> GAMIRSRQPLLDALGVDLPDELLSLALTHRSYAYENGGLPTNERLEFLGDAVLGLTITDALFHRHPDRSEGDLAKLRASVVNTQALADVARRLCAEGLGVHVLLGRGEANTGGADKSSILADGMESLLGAIYLQHGMEKAREVILRLF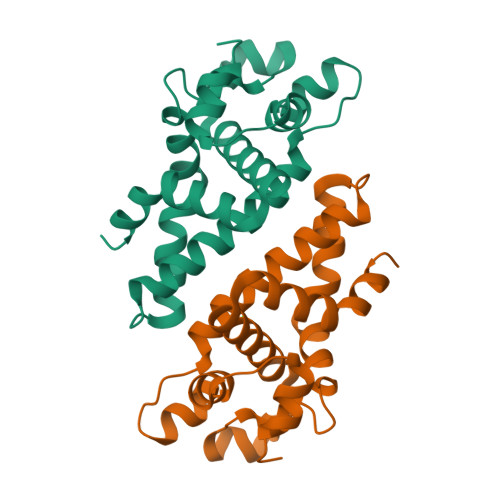GPLLDAAPTLGAGLDWKTSLQELTAARGLGAPSYLVTSTGPDHDKEFTAVVVVMDSEYGSGVGRSKKEAEQKAAAAAWKALEVLDNAMPGKTSA[(3S)-3-amino-3-carboxypropyl](ethyl)methylsulfonium | C7 H16 N O2 S | 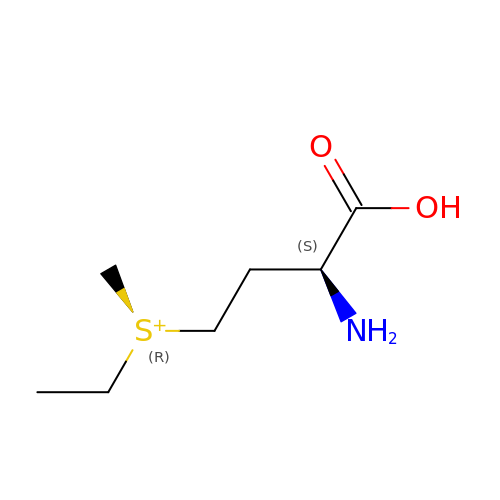CHUUUZMZGJUUGS-UPONEAKYSA-O> GPNTTLVVTTILENPYLMLKGNHQDMEGNDRYEGFCVDMLKELAEILRFNYKIRLVGDGVYGVPEANGTWTGMVGELIARKADLAVAGLTITAEREKVIDFSKPFMTLGISILYRKGTPIESVDDLADQTAIEYGTIHGGSSMTFFQNSRYQTYQRMWNYMYSKQPSVFVKSTEEGIARVLNSNYAFLLESTMNEYYRQRNCNLTQIGGLLDTKGYGIGMPVGSVFR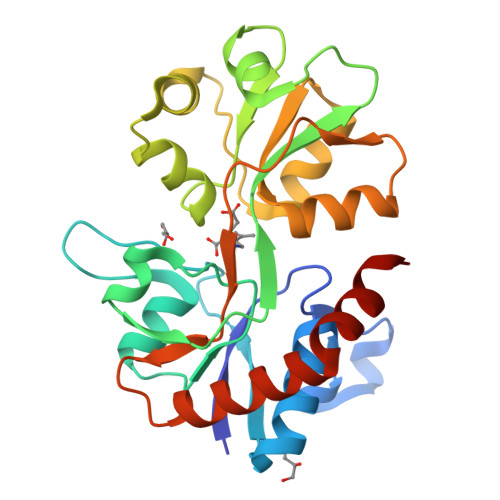DEFDLAILQLQENNRLEILKRKWWEGGKCP>MSGDNGVYSGSAAYNTATAPKVPVSRATFFQNTKSKDFDFKFADGADAIANVLQQMEHGVAQHQLGDMNVRTDGLATVSAVLNGRKRKIANQYMMHFDLFGRAARSTVRMESRIQSFGEGKDVDNFMAKFHNQLSGVYERRSEGVANFGRILATDTDLGGTSGLSVVFNGLLRGLHHVSTVPTPNVANLPIRNNRDGAGAVVGRGDMPGREFMDSSRILPPRSSRWYGAPGQPIVPPAPNNPPAHVAPMETVMAGLQKTVMNELNRVIVSIADVPKLPAHRIRNLIAVLAAVSKPNLGFDANRLEDHSCFTKGWLGFNDILLFPLTVDLFDRVVANEAGVNDAGFIVPNAAPPQFLQNTNQQVIDFRGVGVGQAGDIPALRLAQSWSDAIGFLLDTIGGEAQLAMGLNDMVAQCFHMHGAQTTMLSTPIISRADFGVYHNVVTNMYRRLAYMYTRLIRTNAAAGGGAMLDRQHYQWPTHAKVGFHDDTAVNAAAAAARIHDGLRQPLLDEAFGAGVVQPGNMDLVGAGIDFTRDLTSSLGKAYPEHRPIGADDNKRDLGDFTAGTVDAAASGYEWDNYVYRLFGNMSAMRSKAEFDRLLATFPSSTLSELFIWMGNVGFADTWEERWGYDAAPLCSIPIPAGHDRSMLRNWSWVNVHNVHSVTGTSENVVLAGYVGLSRTHDYIMDTRSTPATSQGRRLAAMFYYTNADKMLSLTFGLAGQLRAAADTTVAKFQICPHTIARAQGYIMTDNDPLSDELKGTDFVTEQFSLAGLTNLYLGYFDGLATRLGIYDLRYTYSEYAECRVELHGIQRNFLTDRLDAFVSYKCLHPIMFEYYMCGANISGGILNGDKAYEQVEMGNIRAYDAMFDTSAARDFNFVGVRGASQQIAAVGGFHIQYKMEVEIQRPGDGTEASRFNVYERYLNNYLRMSDCAPTSVLNAVSPLFWMAGTTRVVLCEAANGYKPMAYDISQTSFWNRENGLWAFTWGESEKTHRPNAIPHGTRRLGNSEVLMNSRFSKILDKKGITKLETRVGGRKRGDNNDDFVAADTRMFIIQDVAGGEHAAYSSLRDPGFALVRAAHTWDTFVQNPRMLLLERGYGNTGFTDTYSAAGIRRTNGHISLRLSALTDDFEFTMHPLARAEYKETSRVSLTSMIYVGTAGKDLSLPTGTVEDIIGAVDGMRRVVRTIGGQTIKTAPVVPPTEQRDMVQEERVGTPVKNAGNANPAADSDNATEGVVEPKN[2x]

Rosellinia necatrix megabirnavirus 1-W779 (RnMBV1) is a non-enveloped icosahedral double-stranded (ds)RNA virus that infects the ascomycete fungus Rosellinia necatrix, a causative agent that induces a lethal plant disease white root rot. RnMBV1 is a potential viro-control approach agent for restraining and controlling the white root rot disease, because the virus can confer hypovirulence to its host fungus. RnMBV1 is an approximately 52 nm bipartite dsRNA mycovirus composed of dsRNA-1 (8.9 kbp in length, AB512282) and dsRNA-2 (7.2 kbp in length, AB512283). The RnMBV1 capsid is composed of 120 chemically identical MCP subunits and additional surface CrPs.

The 3D reconstructions of the full and empty RnMBV1 particles were performed with 12,230 full or 14,602 empty particles, and were then generated with the icosahedral (I) input symmetry. Finally, both maps were generated at an overall resolution of 3.2 Å using the “gold-standard” Fourier shell correlation (FSC) = 0.143 criterion. Each MCP_A proximally surrounds the 5-fold axis, while MCP_B is located distally from the 5-fold and otherwise encompasses the 3-fold capsid intermediates. The amino acid residues Ser2–Lys1193 were modeled for MCP_A, while Ser11–Val1236 were assigned for MCP_B in accordance with the reconstructed full-particle cryo-EM map. In each MCP_B of the RnMBV1 capsid, there is an extra-long 111-amino-acid-residue (Leu1126–Val1236) C-terminal arm/loop, which goes across, interacts, and interlocks with three adjacent subunits in the order of MCP_B1 to A2, A1, B0, whereas that of MCP_A (Leu1126–Lys1193) interacts with only one adjacent subunit. Each full protrusion domain in the RnMBV1 MCP is composed of two fragments of the amino acid residues Ala433–Leu648 and Met965–Ala1125, which form 7 β-strands (Sp-A-G) and 13 α-helices (Hp-A-M). The protrusion domains of MCP_A subunits form dimers on the capsid surface (green rectangle in Fig 3C), while those of MCP_B subunits cluster to build a trimer around each 3-fold axis (yellow triangle in Fig 3C). Hence, for Megabirnaviridae viruses, the pores are also expected to exist; however, the 5-fold pore is obstructed in the RnMBV1 capsid. Positively charged residues Arg140 and Arg141 conformationally block the pore and contribute to positive surface charges.> NEKILIVD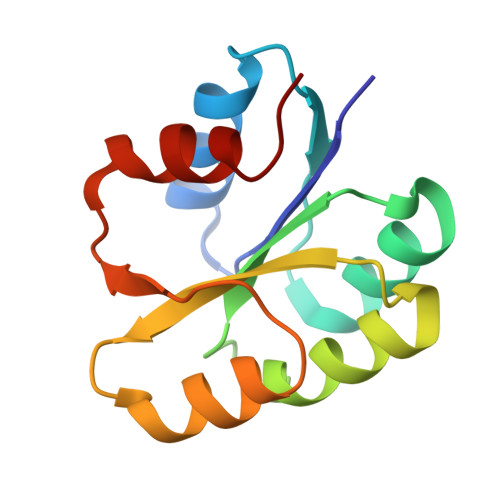DQSGIRILLNEVFNKEGYQTFQAANGLQALDIVTKERPDLVLLDMKIPGMDGIEILKRMKVIDENIRVIIMTAYGELDMIQESKELGALTHFAKPFDIDEIRDAVKKYLPL>[4x]MPVEKHRLDYKPTDFLIDFVDLDFDLYDDRTKVTSTLTMHRREQTPPTDLVLDGEDLELESVELDGNALSMHSTETQKAGDKRVYSLDVDGRLVIAADLLPQEAEKKFKVKTVVYVRPKENLQLMGLYKSGALLVTQCEAEGFRRITYFLDRPDVMSLFKVRLAADEKACPVLLSNGNMVESGKVEGEKGRHFAVFEDPFQKPCYLFALVAGDLKSISQSFTTMSGRNVKVSIFSEPEDSSKLTWALESVLKSMKWDEERFGREYDLDVFNVVC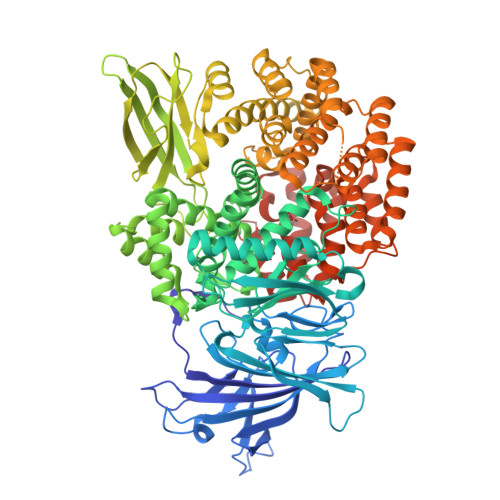AKDFNMGAMENKGLNIFNAALLLADPSTTTDAEYQRILNVVGHEYFHQWTGNRVTCRDWFQLTLKEGLTVFRDQLFTADMCSAAVKRIEDVVFLRSRQFAEDSGPMAHPIRPETYIAMDNFYTATVYDKGAEVIRMYHTLLGEAGFRKGMDLYFKRHDGKAVTCDDFRAAMADANGRDLGQFERWYLQAGTPEVTVSEAVFQPDRKKFKLTLKQRTPPTPGQVEKHPFHIPIKVGLIGKTSKKDILSPPTKVLELTEAEQTFELDAAEDCVLSFLRDFSAPVKVKHEQTDEDIAFLMAHDSDDFAKWQAAHTLASGLLKHRAEQWREKQGEDVEFARLPKIYVEAFKQTLLEQGRDRSIQAYTLRLPDRDGVAQEMEPIDPLALKEATESVRREVGQLLKSDLLKVYASLSAPESEAEESRDQSEVSRRRLRNVILYFLTGERDKEAAALAMNHFKSAKGMTEKYAALSILCDIEGPERTAALEQFYRDAKGDPLVLDKWFAVQALSDVRQVTETVKELQKHADFTAKNPNRLRALIFSFTRNPQFHNKDGAGYALLADSVLAVDRFNPQIAARGAGAFLQWKKYDETRQREMLKQLRRIANAPGLSVDTLEIVQKALAGAPEEATAHHHHHH> MSGCRAQNAPGGIPVTPKSSYSGPIVVDPVTRIEGHLRIEVEVENGKVKNAYSSSTLFRGLEIILKGRDPRDAQHFTQRTCGVCTYTHALASTRCVDNAVGVHIPKNATYIRNLVLGAQYLHDHIVHFYHLHALDFVDVTAALKADPAKAAKVA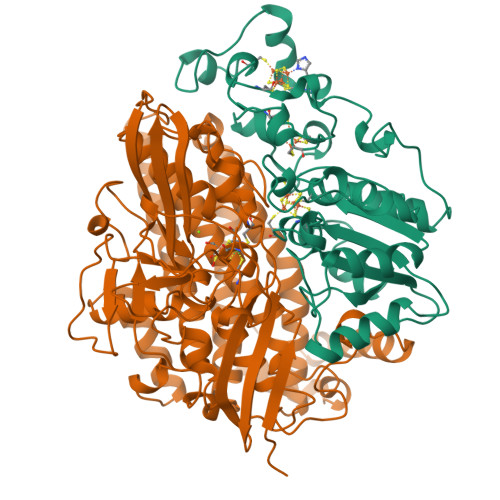SSISPRKTTAADLKAVQDKLKTFVETGQLGPFTNAYFLGGHPAYYLDPETNLIATAHYLEALRLQVKAARAMAVFGAKNPHTQFTVVGGVTCYDALTPQRIAEFEALWKETKAFVDEVYIPDLLVVAAAYKDWTQYGGTDNFITFGEFPKDEYDLNSRFFKPGVVFKRDFKNIKPFDKMQIEEHVRHSWYEGAEARHPWKGQTQPKYTDLHGDDRYSWMKAPRYMGEPMETGPLAQVLIAYSQGHPKVKAVTDAVLAKLGVGPEALFSTLGRTAARGIETAVIAEYVGVMLQEYKDNIAKGDNVICAPWEMPKQAEGVGFVNAPRGGLSHWIRIEDGKIGNFQLVVPSTWTLGPRCDKNNVSPVEASLIGTPVADAKRPVEILRTVHSFDPCIACGVHVIDGHTNEVHKFRIL;> MKISIGLGKEGVEERLAERGVSRRDFLKFCTAIAVTMGMGPAFAPEVARALMGPRRPSVVYLHNAECTGCSESVLRAFEPYIDTLILDTLSLDYHETIMAAAGDAAEAALEQAVNSPHGFIAVVEGGIPTAANGIYGKVANHTMLDICSRILPKAQAVIAYGTCATFGGVQAAKPNPTGAKGVNDALKHLGVKAINIAGCPPNPYNLVGTIVYYLKNKAAPELDSLNRPTMFFGQTVHEQCPRLPHFDAGEFAPSFESEEARKGWCLYELGCKGPVTMNNCPKIKFNQTNWPVDAGHPCIGCSEPDFWDAMTPFYQN>[4x]MRGSHHHHHTTGEDDESECVINYVEK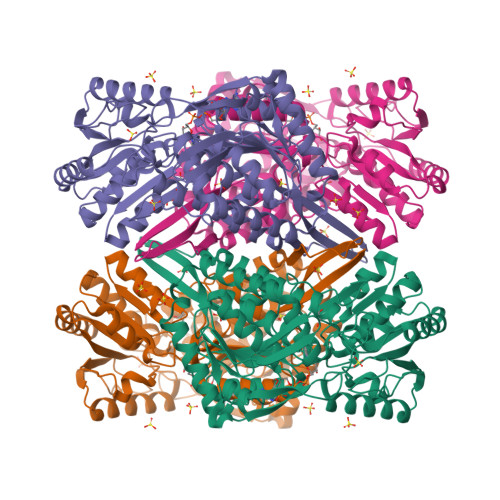AVNKLTLQMPYQLFIGGEFVDAEGSKTYNTINPTDGSVICQVSLAQVSDVDKAVAAAKEAFENGLWGKINARDRGRLLYRLADVMEQHQEELATIEALDAGAVYTLALKTHVGMSIQTFRYFAGWCDKIQGATIPINQARPNRNLTLTKKEPVGVCGIVIPWNYPLMMLSWKTAACLAAGNTVVIKPAQVTPLTALKFAELTLKAGIPKGVVNILPGSGSLVGQRLSDHPDVRKIGFTGSTEVGKHIMKSCALSNVKKVSLELGGKSPLIIFADCDLNKAVQMGMSSVFFNKGENAIAAGRLFVEESIHNQFVQKVVEEVEKMKIGNPLERDTNHGPQNHEAHLRKLVEYCQRGVKEGATLVCGGNQVPRPGFFFQPTVFTDVEDHMYIAKEESFGPIMIISRFADGDVDAVLSRANATEFGLASGVFTRDINKALYVSDKLQAGTVFINTYNKTDVAAPFGGFKQSGFGKDLGEAALNEYLRIKTVTFEY>MPRVLVTGALGQIGTDLSLALRDKFGADSVLVSDVVEPGAKHPLAGLKGVEKLDCLDSNGFEKLVKEFKPTWMYHLPAIMSVRGEAEPDLAMDINVNTTRYALELARKYNIRIFIPSTIAAFGDKCGKTMTKDDTIMNPSTVYGVTKVYTELLGTWYRQKYGVDFRSVRLPGIISAATLPGGGATDYAIHMYHSALLQKKCVCPVLPYESLPMMYMPDTLNSLVKIMEAPLEKLTRTVYNITGFSFSPSELRFSIERCTDRTIEVEYVEGPAQKIANSWPDSLDDSNARNDWGHQV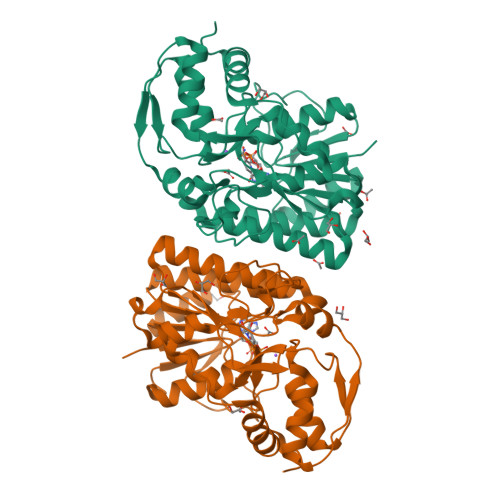KYDIDMMSEDMLRQIPILHGLPSL[2x]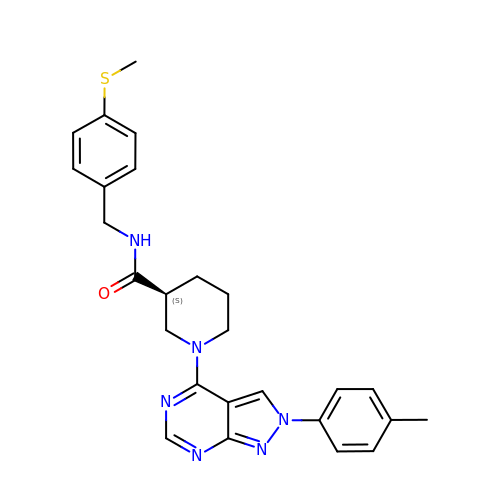(3S)-1-[2-(4-methylphenyl)-2H-pyrazolo[3,4-d]pyrimidin-4-yl]-N-{[4-(methylsulfanyl)phenyl]methyl}piperidine-3-carboxamide | C26 H28 N6 O S | VWUOWUZLQDJSCV-FQEVSTJZSA-N>[4x]ME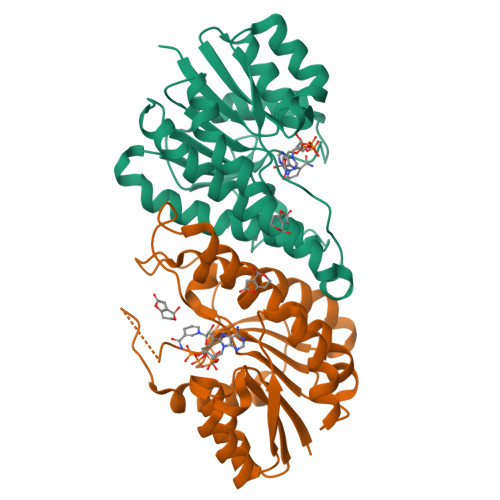QTYFISGANRGIGFSVVQRLAAKSGVKVIATARDPASATALNELAKENPQVKVVQLDISDEESIKKIAKNVSQYTDSIDVFVSNAAIAKSFGPLLNTPREQWIEHFFTNVLGPIRLFQELYPLIKKGTQKKVFFISSNAGSLNLDFGLDFSAFGQSKAALNYSTKELARQLKPENFIVAAVHPGVVTTDMGKGGERAFTAVDEVSAKKFFTPETKITPEESAAALCKLFESLNTTGKYLSYDGTELPW> SDACVHHIKRR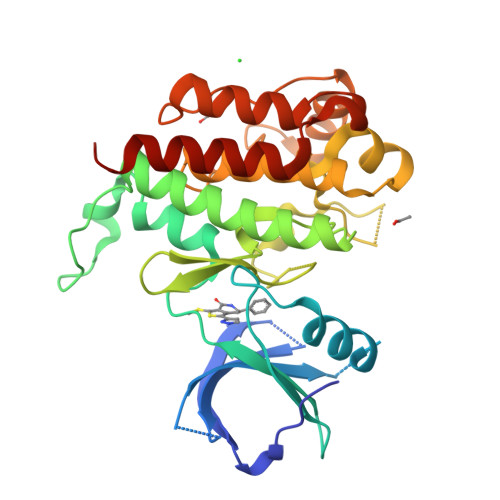DIVLKWELGEGAFGKVFLAECHNLLPEQDKMLVAVKALKEASESARQDFQREAELLTMLQHQHIVRFFGVCTEGRPLLMVFEYMRHGDLNRFLRSHGPDAKLLAGGEDVAPGPLGLGQLLAVASQVAAGMVYLAGLHFVHRDLATRNCLVGQGLVVKIGDFGMSRDIYSTDYYRVGGRTMLPIRWMPPESILYRKFTTESDVWSFGVVLWEIFTYGKQPWYQLSNTEAIDCITQGRELERPRACPPEVYAIMRGCWQREPQQRHSIKDVHARLQALAQAHHHHHH> MGSSHHHHHHSSGENLYFQSHMNVLVIGRGGREHAIAWKAAQSPLVGKLYVAPGNPGIADVAELVHIDELDIEALVQFAKQQAIDLTIVGPEAPLASGIVDRFMAEGLRIFGPSQRAALIEGSKAFAKELMKKYGIPTADHAAFTSYEEAKAYIEQKGAPIVIKADGLAAGKGVTVAQTVEEALAAAKAALVDGQFGTAGSQVVIEEYLEGEEFSFMAFVNGEKVYPLAIAQDHKRAYDGDEGPNTGGMGAYSPVPQISDEMMDAALEAILRPAAKALA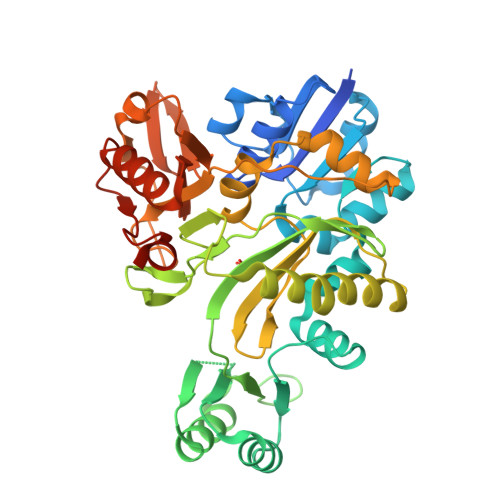AEGRPFLGVLYAGLMATANGPKVIEFNARFGDPEAQVVLPRLKTDLVEAVLAVMDGKELELEWTDEAVLGVVLAAKGYPGAYERGAEIRGLDRISPDALLFHAGTKREGGAWYTNGGRVLLLAAKGETLAKAKEKAYEQLAAIDCDGLFYRRDIGRRAIERASAAYTRMKGR> X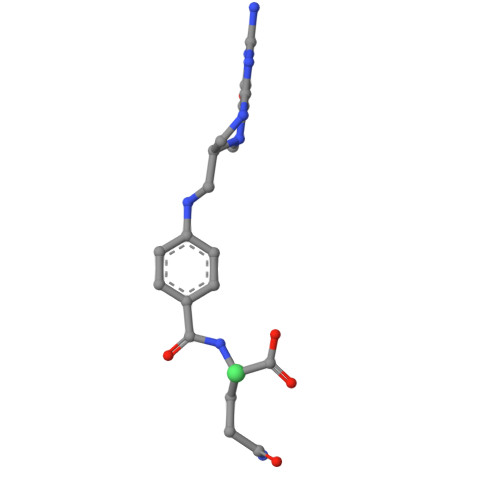EEEEE> GGSMGKTADNHGPVRSETAREGRENQVYSPVTGARLVAGCICLTPDKKQVLMITSSAHKKRWIVPKGGVEKDEPNY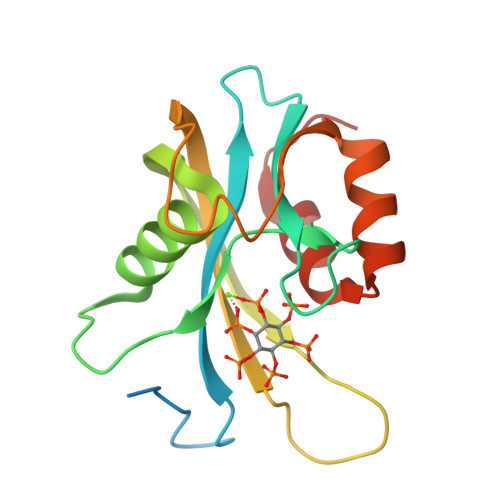ETTAQRETWEEAGCIGKIVANLGTVEDMRPGGGPPRTEFHFYELEIENLLDKFPECHKRHRKLYSYTEAKQNLIDAKRPELLEALNRSAIIKDDK> MGPLVARDAATILSDLSTIKTDINTLTQHFNEFTGDLLQALAAQAVEQQLESDIDQATADAK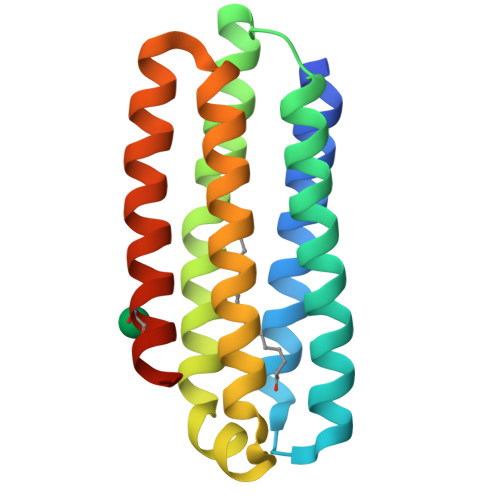ATSALSAADSTSVTNALLGLKPDIVTSLDAIVAKKPQVDSAGVGSLVLSDLNALQSKTDALSGALQDIATATDKDTIASGTQDIDAAFSSAIAVFSHHHHHH> GPLGSMAHAGRTGYDNREIVMKYIHYKLSQRGY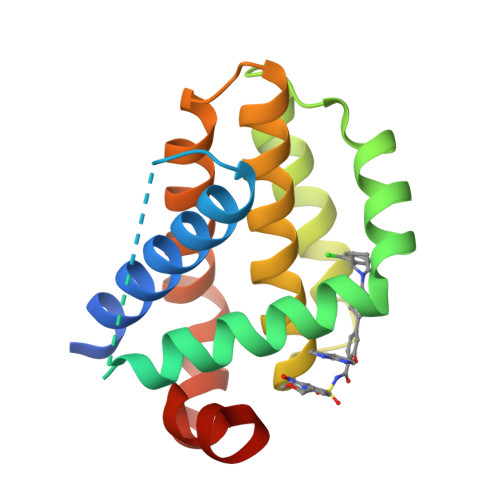EWDAGDDVEENRTEAPEGTESEVVHLTLRQAGDDFSRRYRRDFAEMSSQLHLTPFTARGRFATVVEELFRDGVNWGRIVAFFEFGGVMCVESVNREMSPLVDNIALWMTEYLNRHLHTWIQDNGGWDAFVELYGPSMR>[14x]NLIPTVIEQTNRGERAYDIYSRLLKDRIIMLGSAIDDNVANSIV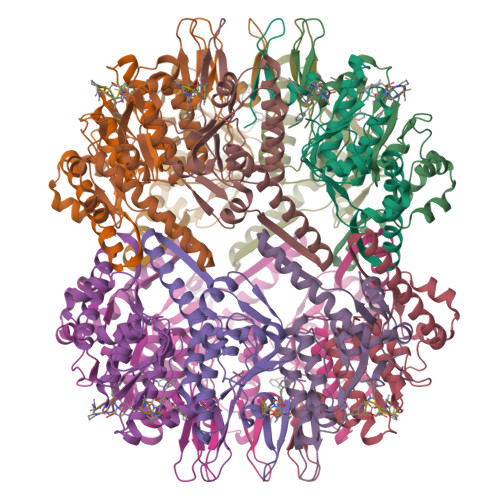SQLLFLAAEDPEKEISLYINSPGGSITAGMAIYDTMQFIKPKVSTICIGMAASMGAFLLAAGEKGKRYALPNSEVMIHQPLGGAQGQATEIEIAAKRILLLRDKLNKVLAERTGQPLEVIERDTDRDNFKSAEEALEYGLIDKILTHTEDKKHHHHHH;>[14x]XFSPAAP5-(4-methylpiperazin-1-yl)-2-phenylmethoxy-~{N}-pyridin-3-yl-benzamide | C24 H26 N4 O2 | 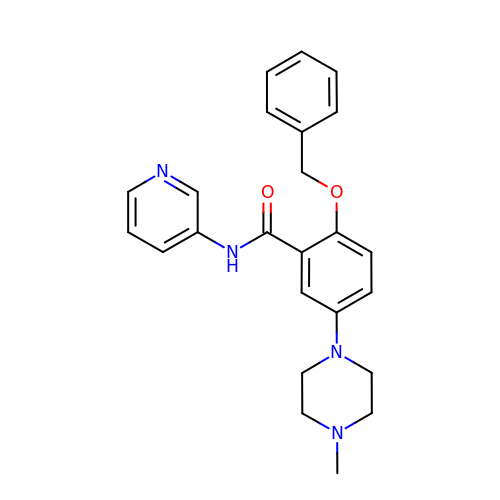QGEBKIOJSNPDFE-UHFFFAOYSA-N>DYKDDDDKGSGSGIAELPPKVSVFVPPRDGFFGNPRKSKLICQATGFSPRQIQVSWLREGKQVGSGVTTDQVQAEAKESGPTTYKVTSTLTIKESDWLSQSMFTCRVDHRGLTFQQNASSMCVPDQDTAIRVFAIPPSFASIFLTKSTKLTCLVTDLTTYDSVTISWTRQNGEAVKTHTNISESHPNATFSAVGEASICEDDWNSGERFTCTVTHTDLPSPLKQTISRPKGVALHRPDVYLLPPAREQLNLRESATITCLVTGFSPADVFVQWMQRGQPLSPEKYVTSAPMPEPQAPGRYFAHSILTVSEEEWNTGETYTCVVAHEALPNRVTERTVDKSTGKPTLYNVSLVMSDTAGTCY[10x];> MKNHLLFWGVLAVFIKAVHVKAQEDERIVLVDNKCKCARITSRIIRSSEDPNEDIVERNIRIIVPLNNRENISDPTSPLRTRFVYHLSDLCKKCDPTEVELDNQIVTATQSNICDEDSATETCYTYDRNKCYTAVVPLVYGGETKMVETALTPDACYPDEQKLISEEDL;> SPSGVRLVGGLHRCEGRVEVEQKGQWGTVCDDGWDIKDVAVLCRELGCGAASGTPSGILYEPPAEKEQKVLIQSVSCTGTEDTLAQCEQEEVYDCSHDEDAGASCENPESSFSPVPEGVRLADGPGHCKGRVEVKHQNQWYTVCQTGWSLRAAKVVCRQLGCGRAVLTQKRCNKHAYGRKPIWLSQMSCSGREATLQDCPSGPWGKNTCNHDEDTWVECEDPFDLRLVGGDNLCSGRLEVLHKGVWGSVCDDNWGEKEDQVVCKQLGCGKSLSPSFRDRKCYGPGVGRIWLDNVRCSGEEQSLEQCQHRFWGFHDCTHQEDVAVICSG

Apoptosis inhibitor of macrophage (AIM/CD5L) is a soluble protein belonging to the scavenger receptor cysteine-rich (SRCR) superfamily that contributes to prevention of a wide range of diseases associated with infection, inflammation, and cancer. AIM forms complexes with IgM pentamers which helps maintain high-levels of circulating AIM in serum for subsequent activation on release from the complex. Here we apply cryogenic electron microscopy imaging (cryo-EM) to show how interfaces on both of AIM’s C-terminal SRCR domains interact with the Fcμ constant region and J chain components of the IgM core. The human Fcμ/J/AIM complex shows the binding of tandem AIM SRCR domains to IgM leading to sequestration and stabilisation of AIM.

We expressed human pentameric IgM core which includes ten copies of Fcμ chains from Cμ2 to the C-terminal tailpiece and one J chain, as well as full-length human AIM (hAIM). As published previously, the density of the cryo-EM map of pentameric IgM core contains ten Cμ3 and Cμ4 domains (in grey) and a single J chain (in orange), with the absence of Cμ2 domains which are disordered in the map due to their flexible linkage. AIM engages pentameric IgM core with 1:1 stoichiometry. AIM (in cyan) occupies a groove of Fcμ/J, with SRCR2 and SRCR3 domains proximal to the J chain and subunit Fcμ5. The global map resolution is 3.6 Å, with local resolution at the interface predominantly ranging from 3 Å to 3.5 Å. The density of the N-terminal SRCR1 domain appears only at lower contour level, indicating a flexible connection to SRCR2. Comparison of the Fcμ/J/AIM to other pentameric IgM structures suggests that only minor changes in the IgM core occur on AIM binding, but nevertheless AIM binding has functional consequences for IgM. Polymeric immunoglobulin receptor (pIgR), a component of secretory IgM which mediates the IgM transcytosis through the mucosal epithelial cells, also occupies the cleft in the IgM pentamer when bound, and therefore pIgR and AIM cannot bind IgM at the same time. Superposition of the Fcμ/J/AIM complex on the IgM/FcμR structure, shows that Fcμ/J/AIM can accommodate binding of all eight FcμR Ig domains without clashes. Similarly, it has also been reported that AIM does not influence complement pathway activation, consistent with our Fcμ/J/AIM structure as the binding sites on IgM for C1q are at the tips of Cμ3 domains which are distant from AIM.> MESVAAESAPAPENEHSQETPESNSSVYTTFMKSHRCYDLIPTSSKLVVFDTSLQVKKAFFALVTNGVRAAPLWDSKKQSFVGMLTITDFINILHRYYKSALVQIYELEEHKIETWREVYLQDSFKPLVCISPNASLFDAVSSLIRNKIHRLPVIDPESGNTLYILTHKRILKFLKLFITEFPKPEFMSKSLEELQIGTYANIAMVRTTTPVYVALGIFVQHRVSALPVVDEKGRVVDIYSKFD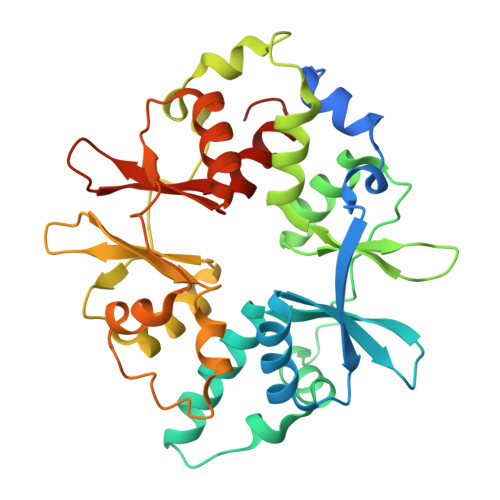VINLAAEKTYNNLDVSVTKALQHRSHYFEGVLKCYLHETLEAIINRLVEAEVHRLVVVDEHDVVKGIVSLSDILQALVLTGGEKKP>[2x]GDITHMAPSRKFFVGGNWMMNGRKQSLGELIGTLNAAKVPADTEVVCAPPTAYIDFARQKLD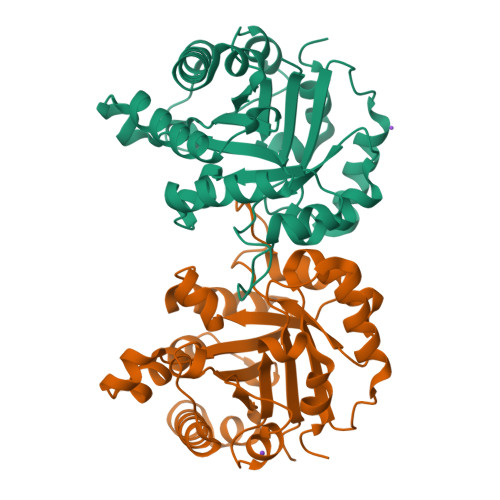PKIAVAAQNCYKVTNGAFTGEISPGMIKDCGATWVVLGHSERRHVFGESDELIGQKVAHALAEGLGVIACIGEKLDEREAGITEKVVFEQTKVIADNVKDWSKVVLAYEPVWAIGTGKTATPQQAQEVHEKLRGWLKSNVSDAVAQSTRIIYGGSVTGATCKELASQPDVDGFLVGGASLKPEFVDIINAKQ>[2x]MHHHHHHEPLILTAAITGAETTRADQPNLPITPEEQAKEAKACFEAGARVIHLHIREDDGRPSQRLDRFQEAISAIREVVPEIIIQISTGGAVGESFDKRLAPLALKPEMATLNAGTLNFGDDIFI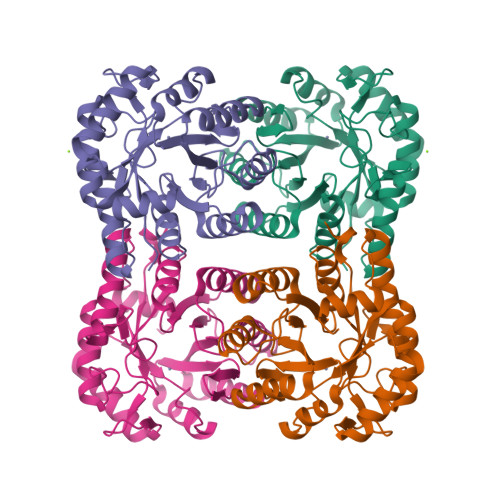NHPADIIRLAEAFKQYNVVPEVEVYESGMVDAVARLIKKGIITQNPLHIQFVLGVPGGMSGKPKNLMYMMEHLKEEIPTATWAVAGIGRWHIPTSLIAMVTGGHIRCGFEDNIFYHKGVIAESNAQLVARLARIAKEIGRPLATPEQAREILALNK> MSVLISGASGYIAKHIVRVLLEQNYKVIGTVRSQDIADKLLKQYNNPNLSYEIVPEIANLDAF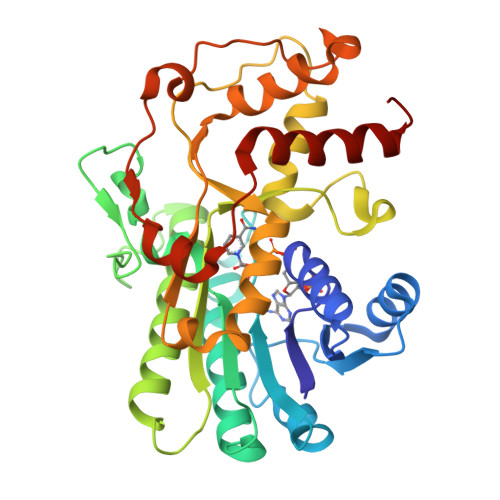DDIFKKHGKEIKYVIHAASPVNFGAKDLEKDLVIPAINGTKNMFEAIKKYAPDTVERVVMTASYASIMDPHRQNDPTLTLDEETWNPVTEENAYEDVFTAYCASKTFAEKEAWKFVKENSDAVKFKLTTIHPSFVFGPQNFDEDVTEKLNETCEIINGLLHAPFDTKVEKTHFSQFIDVRDVAKAHVLGFQKDELINQRLLLCNGAFSLQDIVNVFNEDFPELKGQFPPEDKDTDLNKGVTGCKIDNEKTKKLLAFEFTPFHKTIHDTVYQILHKEGRV> RTFSYTLEDHTKQAFGIMNELRLSQQLCDVTLQVKYQDAPAAQFMAHKVV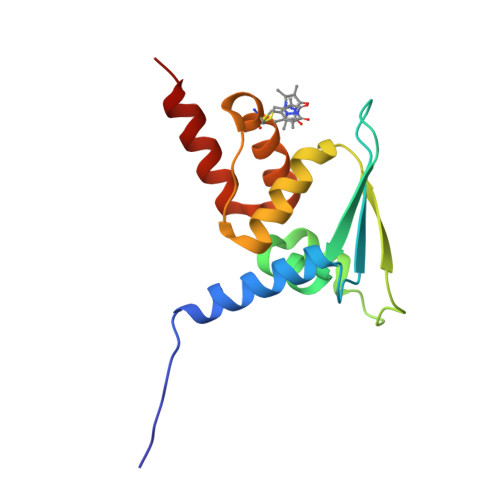LASSSPVFKAMFTNGLREQGMEVVSIEGIHPKVMERLIEFAYTASISMGEKCVLHVMNGAVMYQIDSVVRACADFLVQQLD>[2x]TPHALLLISIDGLRADMLDRGITPNLSHLAREGVRARWMAPSYPSLTFPNHYTLVTGLRPDHHGIVHNSMRDPTLG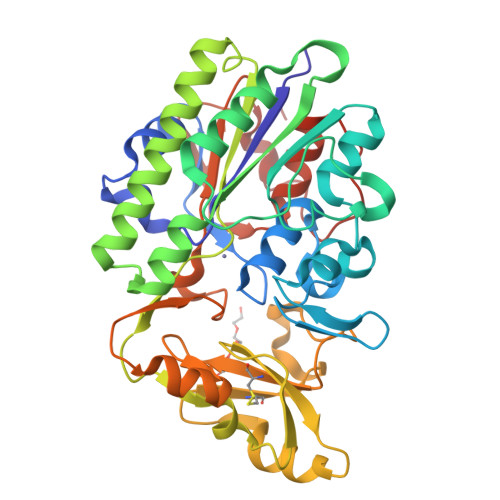GFWLSKSEAVGDARWWGGEPVWVGVENTGQHAATWSWPGSEAAIKGVRPSQWRHYQKGVRLDTRVDAVRGWLATDGAQRNRLVTLYFEHVDEAGADHGPESRQYADAVRAVDAAIGRLLAGMQRDGTRARTNIIVVSDHGMAEVAPGHAISVEDIAPPQIATAITDGQVIGFEPLPGQQAAAEASVLGAHDHYDCWRKAELPARWQYGSHPRIPSLVCQMHEGWDALFPDKLAKRAQRGTRGSHGYDPALPSMRAVFLAQGPDLAQGKTLPGFDNVDVYALMSRLLGIPAAPNDGNPATLLPALRMP>[2x]TEVLWPAVPNGTDAAFLAGPGSSWGNSTVA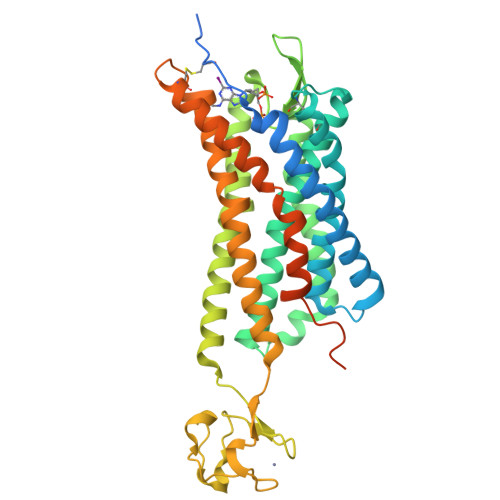STAAVSSSFKCALTKTGFQFYYLPAVYILVFIIGFLGNSVAIWMFVFHMKPWSGISVYMFNLALADFLYVLTLPALIFYYFNKTDWIFGDAMCKLQRFIFHVNLYGSILFLTCISAHRYSGVVYPLKSLGRLKKKNAICISVLVWLIVVVAISPILFYSGTGVRKNKTITCYDTTSDEYLRSYFIYSMCTTVAMFCVPLVLILGCYGLIVRALIYKMKKYTCTVCGYIYNPEDGDPDNGVNPGTDFKDIPDDWVCPLCGVGKDQFEEVEEPLRRKSIYLVIIVLTVFAVSYIPFHVMKTMNLRARLDFQTPAMCAFNDRVYATYQVTRGLASLNSCVNPILYFLAGDTFRRRLSRATRKASRRSEANLQSKSEDMTLNILPEFKQNGDTSL> GDPVEDIIHDALGSTARRAISSATNVESAANTTPSSHRLETGRVPALQAAETGATSNATDENMIETRCVVNRNGVLETTINHFFSRSGLVGVVNLTDGGTDTTGYVTWDIDIMGFVQLRRKCEMFTYMRFNAEFTFVTTTKNGEARPYMLQYMYVPPGAPKPTGRDAFQWQTATNPSVFVKLTDPPAQVSVPFMSPASAYQWFYDGYPTFGQHPETSNTTYGLCPNNMMGTFAVRVVSREASQLKLQTRVYMKLKHVRAWVPRPIRSQPYLLKNFPNYDSSKITNSARDRSSIKQAN;> SPSVEACGYSDRVAQLTVGNSSITTQEAANIVLAYGEWPEY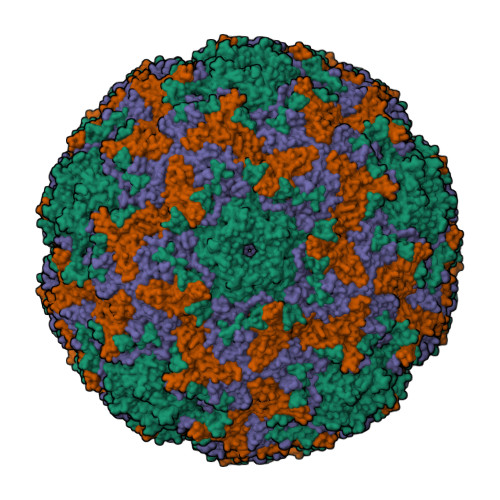CPDTDATAVDKPTRPDVSVNRFYTLDSKMWQENSTGWYWKFPDVLNKTGVFGQNAQFHYLYRSGFCLHVQCNASKFHQGALLVAVIPEFVIAGRGSNTKPNEAPHPGFTTTFPGTTGATFHDPYVLDSGVPLSQALIYPHQWINLRTNNCATVIVPYINAVPFDSAINHSNFGLIVIPVSPLKYSSGATTAIPITITIAPLNSEFGGLRQAVSQ;> GIPAELRPGTNQFLTTDDDTAAPILPGFTPTPTIHIPGEVHSLLELCRVETILEVNNTTEATGLTRLLIPVSSQNKADELCAAFMVDPGRIGPWQSTLVGQICRYYTQWSGSLKVTFMFTGSFMATGKMLVAYSPPGSAQPANRETAMLGTHVIWDFGLQSSVSLVIPWISNTHFRTAKTGGNYDYYTAGVVTLWYQTNYVVPPETPGEAYIIAMGADLYKFTLKICKDTDEVTQQAVLQ;> MGAQVSTQKSGSHETGNVATGGSTINFTNINYYKDSYAASATRQDFTQDPKKFTQPVLDSIRELSAPLN>[2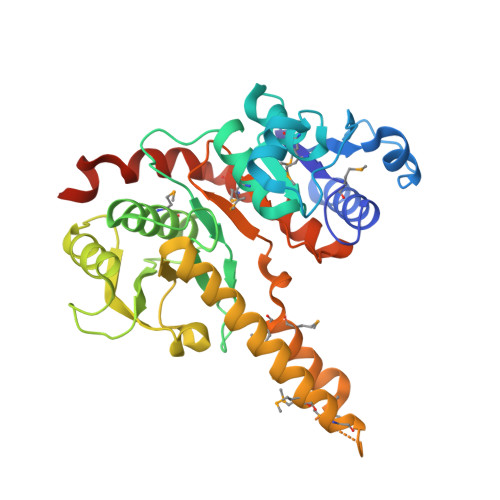x]MSLRIAVDAMGGDHAPKAVIDGVIKGIEAFDDLHITLVGDKTTIESHLTTTSDRITVLHADEVIEPTDEPVRAVRRKKNSSMVLMAQEVAENRADACISAGNTGALMTAGLFIVGRIKGIDRPALAPTLPTVSGDGFLLLDVGANVDAKPEHLVQYAIMGSVYSQQVRGVTSPRVGLLNVGTEDKKGNELTKQTFQILKETANINFIGNVEARDLLDDVADVVVTDGFTGNVTLKTLEGSALSIFKMMRDVMTSTLTSKLAAAVLKPKLKEMKMKMEYSNYGGASLFGLKAPVIKAHGSSDSNAVFRAIRQAREMVSQNVAALIQEEVKEEKTDEEGGSHHHHHH>MQNVGFIGWRGMVGSVLMQRMVEERDFDAIRPVFFSTSQLGQAAPSFGGTTGTLQDAFDLEALKALDIIVTCQGGDYTNEIYPKLRESGWQGYWIDAASSLRMKDDAIIILDPVNQDVITDGLNNGIRTFVGGNCTVSLMLMSLGGLFANDLVDWVSVATYQAASGGGARHMRELLTQMGHLYGHVADELATPSSAILDIERKVTTLTRSGELPVDNFGVPLAGSLIPWIDKQLDNGQS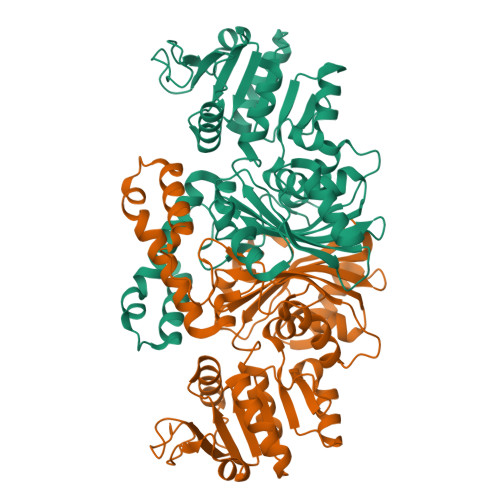REEWKGQAETNKILNTSSVIPVDGLCVRVGALRCHSQAFTIKLKKDVSIPTVEELLAAHNPWAKVVPNDREITMRELTPAAVTGTLTTPVGRLRKLNMGPEFLSAFTVGDQLLWGAAEPLRRMLRQLA[3x]> MQEPLAAGAVILRRFAFNAAEQLIRDINDVASQSPFRQMVTPGGYTMSVAMT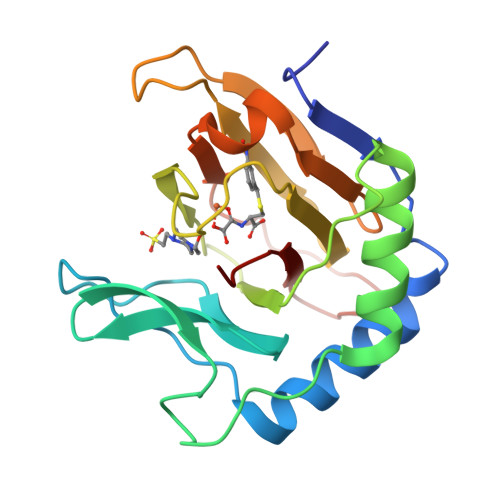NCGHLGWTTHRQGYLYSPIDPQTNKPWPAMPQSFHNLCQRAATAAGYPDFQPDACLINRYAPGAKLSLHQDKDEPDLRAPIVSVSLGLPAIFQFGGLKRNDPLKRLLLEHGDVVVWGGESRLFYHGIQPLKAGFHPLTIDCRYNLTFRQAGKKE4-({5-fluoro-4-[2-methyl-1-(propan-2-yl)-1H-imidazol-5-yl]pyrimidin-2-yl}amino)-N-[2-(piperidin-1-yl)ethyl]benzamide 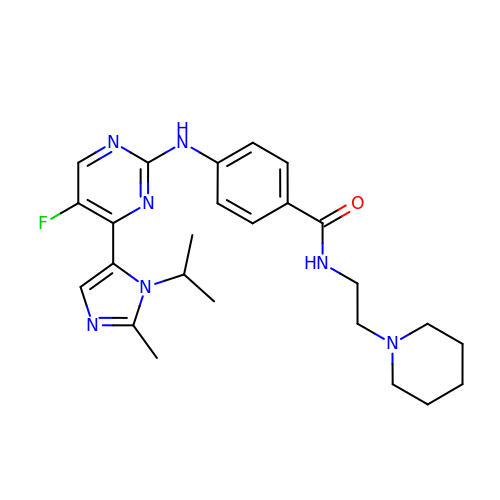| C25 H32 F N7 O | PGXDTVQNUCGXDO-UHFFFAOYSA-N>LQGRIAASADAQLELIGPRAAAAASLESAVLH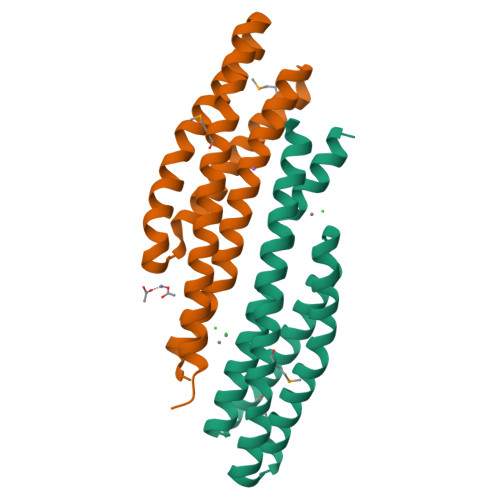VSLTARAYALTPEPARMDALQAALRRLEGAAARFAALPKSPEGAALSGRILAAVPPFEKAAVALGTAVATGGDDSAIRAREATLPPMREELLSLLRTFGALQQAHDAGASHTILAYQRDT[2x]hydrolyzed ceftazidime | C22 H25 N6 O8 S2 | 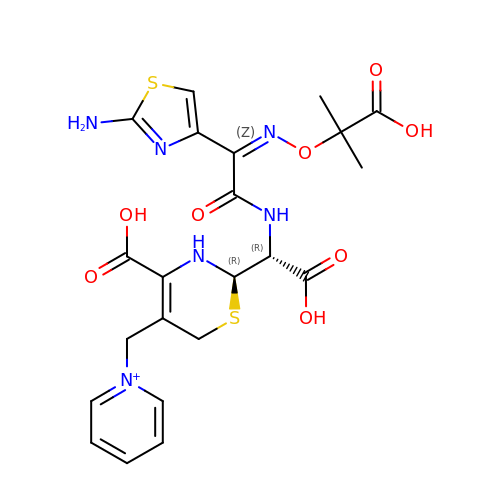ZFKSAQZBKJRFHB-NUYJMBSPSA-O> STKNGIIELEQETEEELEQNQEIDYSNYPEFSWDTMPLYMHVRKNTAYTDEEINYLASFPLITLEKSQAQNTYGSTEEGTLAT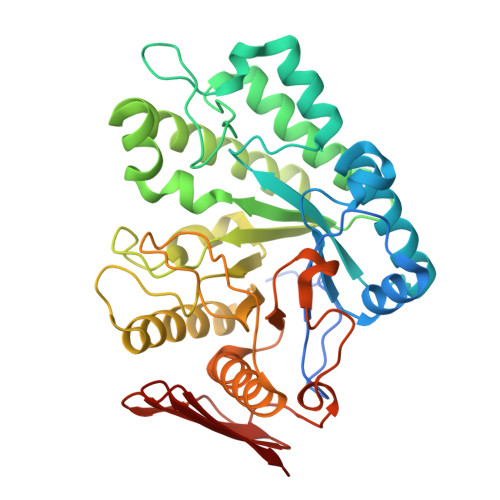ASAIKLKNNKAKVLYYRNVVINWGNYKNDDEFISKNPSALLKNQNNELVYMPNGSTPFFDITKSFVQEYWLKSVEDMVATPNIDGTFIDANIKVLVPSFFSSKVGVNKQAEIENSYFSMMSRLKESLSNNLILANIIRVRPEFEENGLEYLGYFNGSYLEGFDSEAFGMSNAEYLVEGIEATQKAAQSGKIITMTLGLGEAIDNNTGIDDQREDVDLNDEELNKRVDYLLAIFLICAEKYSYVYLHDGYLATNSAVWLHQFDQYKKALGAPLGKAIKNGYIYTRKFENLDVWLNLETQTATLTWKE>[2x]GPMKTEMKDDFAKLEEQFDAKLGIFALDTGTNRTVAYRPDERFAFASTIKALTVGVLLQQKSIEDLNQRITYTRDDLVNYNPITEKHVDTGMTLKELADASLRYSDNAAQNLILKQIGGPESLKKELRKIGDEVTNPERFSPELNEVNPGETQD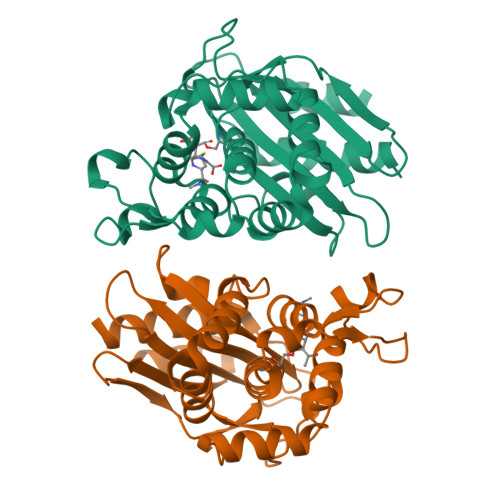TSTARALVTSLRAFALEDKLPSEKRELLIDWMKRNTTGDALIRAGVPDGWEVADKTGAASYGTRNDIAIIWPPKGDPVVLAVLSSRDKKDAKYDDKLIAEATKVVMKALNMNGK> AAVPFEERVKIFQRLIYADKQEVQGDGPFLDGINVTIRRNYIYEDAYDKLSPENEPDLKKR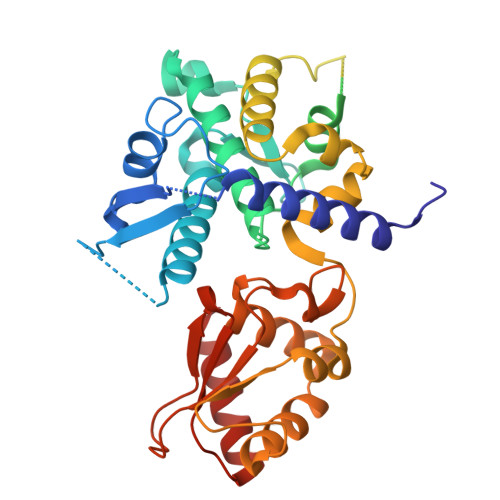IRVHLLNAHGLDEAGIDGGGIFREFLNELLKSGFNPNQGFFKTTNEGLLYPNPAAQMLVGDSFARHYYFLGRMLGKALYENMLVELPFAGFFLSKLLGTSADVDIHHLASLDPEVYKNLLFLKSYEDDVEELGLNFTVVNNDLGEAQVVELKFGGKDIPVTSANRIAYIHLVADYRLNRQIRQHCLAFRQGLANVVSLEWLRMFDQQEIQVLISGAQVPISLEDLKSFTNYSGGYSADHPVIKVFWRVVEGFTDEEKRKLLKFVTSCSRPPLLGFKELYPAFCIHNGGSDLERLPTASTCMNLLKLPEFYDETLLRSKLLYAIECAAGFELS> NPVIA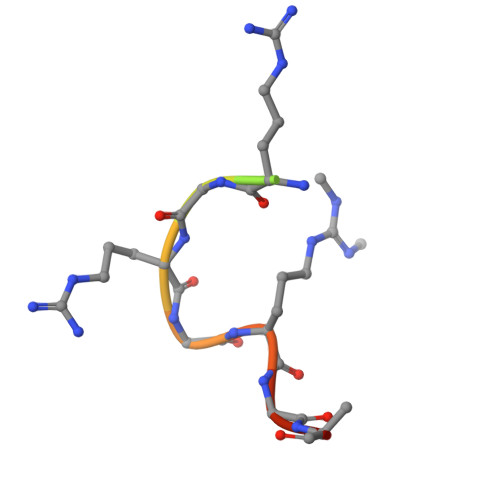RGRGRGRK> MSVYPKALRDEYIMSKTLGSGACGEVKLAFERKTCKKVAIKIISKRKFAIGSAREADPALNVETEIEILKKLNHPCIIKIKNFFDAEDYYIVLELMEGGELFDKVVGNKRLKEATCKLYFYQMLLAVQYLHENGIIHRDLKPENVLLSSQEEDCLIKITDFGHSKILGETSLMRTLCGTPTYLAPEVLVSVGTAGYNRAVDCWSLGVILFICLSGYPPFSEHRTQVSLKDQITSGKYNFIPEVWAEVSEKALDLVKKLLVVDPKARFTTEEALRHPWLQDEDMKRKFQDLLSEENESTA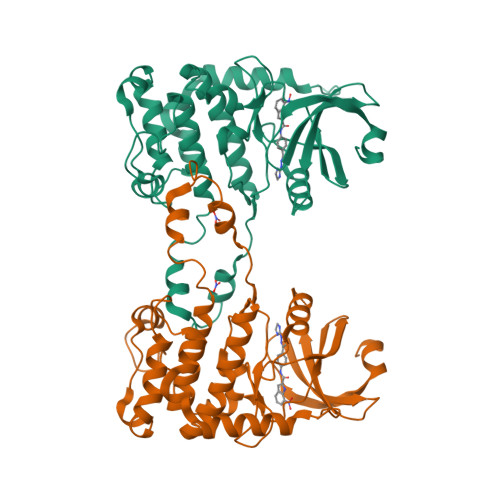LPQVLAQPSTSRKRPREGEAEGAE> RYNDYKLDFRRQQMQDFFLAHKDEEWFRSKYHPDEVGKRRQEARGALQNRLRVFLSLMETGWFDNLLLDIDKADAIVKMLDAAVIKMEGGTENDLRILEQ;> GLECKPRPLHKTCSLFMRNIAPNISRAEIISLCKRYPGFMRVALSEPQPERRFFRRGWVTFDRSVNIKEICWNLQNIRLRECELSPGVNRDLTRRVRNINGITQHKQIVRNDIKLAAKLIHTLDDRTQLWASEPGTPPLPTSLPSQNPILKNITDYLIEEVSAEEEELLGS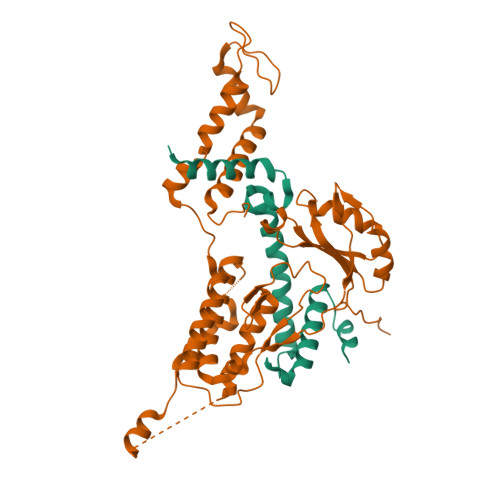SGGAPPEEPPKEGNPAEINVERDEKLIKVLDKLLLYLRIVHSLDYYNTCEYPNEDEMPNRCGIIHVRGPMPPNRISHGEVLEWQKTFEEKLTPLLSVRESLSEEEAQKMGRKDPEQEVEKFVTSNTQELGKDKWLCPLSGKKFKGPEFVRKHIFNKHAEKIEEVKKEVAFFNNFLTDAKRPALPE> GPLGSASGEGKKVDIAGIYPPVTTPFTATAEVDYGKLEENLHKLGTFPFRGFVVQGSNGEFPFLTSSERLEVVSRVRQAMPKNRLLLAGSGCESTQATVEMTVSMAQVGADAAMVVTPCYYRGRMSSAALIHHYTKVADLSPIPVVLYSVPANTGLD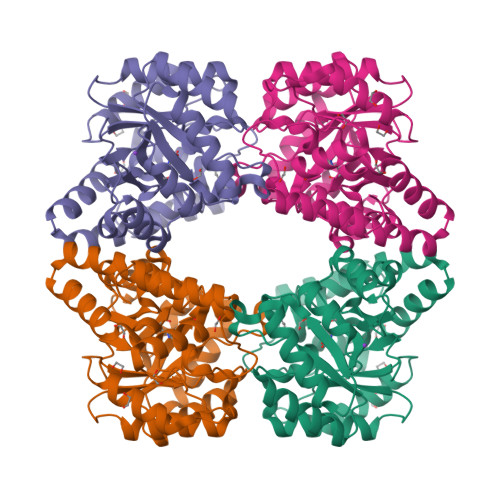LPVDAVVTLSQHPNIVGMKDSGGDVTRIGLIVHKTRKQDFQVLAGSAGFLMASYALGAVGGVCALANVLGAQVCQLERLCCTGQWEDAQKLQHRLIEPNAAVTRRFGIPGLKKIMDWFGYYGGPCRAPLQELSPAEEEALRMDFTSNGWL>[2x]KKSIPVRGAAIFNENLSKILLVQGTESDSWSFPRGKIS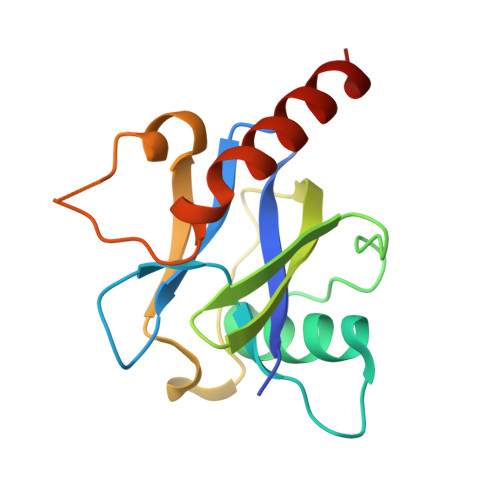KDENDIDCCIREVKEEIGFDLTDYIDDNQFIERNIQGKNYKIFLISGVSEVFNFKPQVRNQIDKIEWFDFKKISKTMYKSNIKYYLINSMMRPLSMWLRHQRQIKNED>MEGNTILKIVLICTILAGLFGQVVPVYAENTTYQTPTGIYYEVRGDTIYMINVTSGEETPIHLFGVNWFGFETPNHVVHGLWKRNWEDMLLQIKSLGFNAIRLPFCTESVKPGTQPIGIDYSKNPDLRGLDSLQIMEKIIKKAGDLGIFVLLDYHRIGCTHIEPLWYTEDFSEEDFINTWIEVAKRFGKYWNVIGADLKNEPHSVTSPPAAYTDGTGATWGMGNPATDWNLAAERIGKAILKVAPHWLIFVEGTQFTNPKTDSSYKWGYNAWWGGNLMAVKDYPVNLPRNKLVYSPHVYGPDVYNQPYFGPAKGFPDNLPDIWYHHFGYVKLELGYSVVIGAFGGKYGHGGDPRDVIWQNKLVDWMIENKFCDFFYW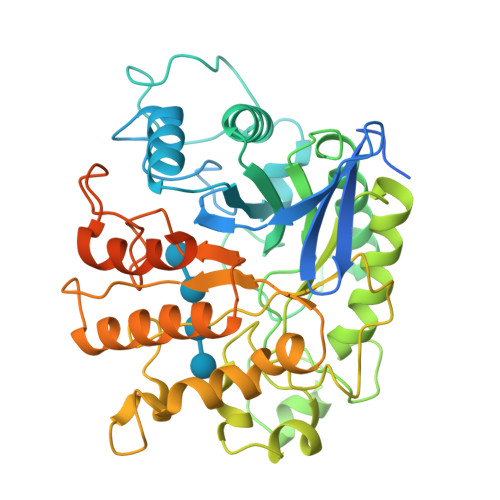SWNPDSGDTGGILQDDWTTIWEDKYNNLKRLMDSCSKSSSSTQSVIRSTTPTKSNTSKKICGPAILIILAVFSLLLRRAPR[3x]>[2x]EQTAAPAKPVTVEAKNETFAPQHPDQYLSWKATSEQSERVDALAEDPRLVILWAGYPFSRDYN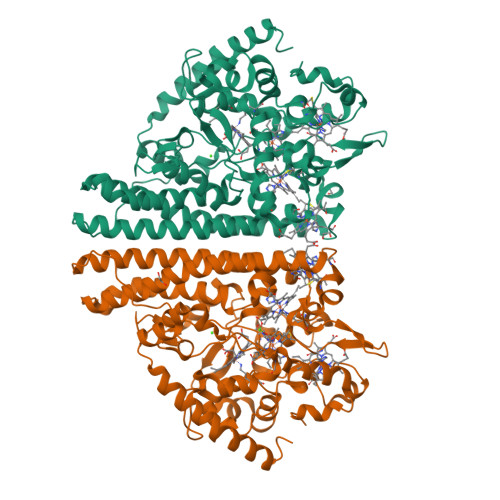KPRGHAFAVTDVRETLRTGAPKNAEDGPLPMACWSCKSPDVARLIQKDGEDGYFHGKWARGGPEIVNNLGCADCHNTASPEFAKGKPELTLSRPYAARAMEAIGKPFEKAGRFDQQSMVCGQCHVEYYFDGKNKAVKFPWDDGMKVENMEQYYDKIAFSDWTNSLSKTPMLKAQNPEYETWTAGIHGKNNVTCIDCHMPKVQNAEGKLYTDHKIGNPFDNFAQTCANCHTQDKAALQKVVAERKQSINDLKIKVEDQLVHAHFEAKAALDAGATEAEMKPIQDDIRHAQWRWDLAIASHGIHMHAPEEGLRMLGTAMDKAADARTKLARLLATKGITHEIQIPDISTKEKAQQAIGLNMEQIKAEKQDFIKTVIPQWEEQARKNGLLSQ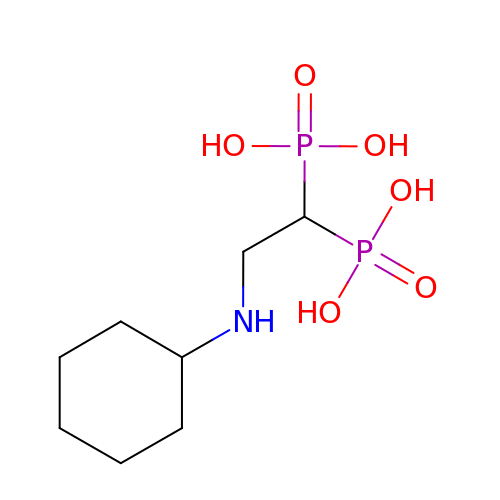[2-(cyclohexylamino)ethane-1,1-diyl]bisphosphonic acid | C8 H19 N O6 P2 | OAHUDYBQKIUBMC-UHFFFAOYSA-N> MSHHHHHHVSKIFFEQGTYQCLENCGTVALTIIRRGGDLTNTVFVDFRTEDGTANAGSDYEFTEGTVVFKPGETQKEIRVGIIDDDIFEEDKNFLVHLSNVKVSSEASEDGILEANHVSALACLGSPSTATVTIFDDDHAGIFTFEEPVTHVSESIGIMEVKVLRTSGARGNVIVPYKTIEGTARGGGEDFEDTCGELEFQNDEIVKTISVKVIDDEEYEKNKTFFLEIGEPRLVEMSEKKGGFTITEEYDDKQPLTSKEEEERRIAEMGRPILGEHTKLEVIIEESYEFKSTVD

In contrast, the eukaryotic NCX has evolved an allosteric Ca2+ regulatory element encoded by a large cytosolic domain (∼500 amino acids) between transmembrane helices 5 and 6 i.e. the repeated membrane motif, designated as f-loop. This large loop includes two Ca2+-binding regulatory domains (CBD1 and CBD2), connected by a short linker. High-resolution NMR and crystal structures of isolated CBD1 and CBD2 domains of eukaryotic NCX revealed four Ca2+ sites (Ca1-Ca4) on CBD1 and two Ca2+ sites (CaI-CaII) on CBD2. Different lines of evidence suggest that CBD2 interacts with CBD1 to modify the equilibrium and kinetic properties of the primary Ca2+ sensor (Ca3-Ca4 sites), either in isolated CBD12 or in intact NCX.

To test this working hypothesis, we crystallized and determined the crystal structure of a two-domain CBD12 tandem from the brain splice variant (NCX1.4). In order to crystallize the tandem, we employed a previously characterized mutant, E454K. (i) The E454K substitution replaces the Ca2+ ion at Ca1 site of CBD1, thus, stabilizing the protein’s structure through a charge compensation mechanism. The overall structure of CBD12-E454K shows two nearly identical CBD domains, each composed of an anti-parallel β-sandwich, with root mean square deviation (r.m.s.d for 109 Cα atoms) of 1.3 Å. In agreement with the previously published crystal structure of CBD1-E454K, our structure reveals three Ca2+ ions in CBD1 that correspond to Ca2, Ca3 and Ca4 in CBD1-WT. Notably, there is no indication for bound Ca2+ ions in CBD2 of our structure. We ascribe the lack of bound Ca2+ in CBD2 to crystal packing between symmetry mates. The interface involves mainly interactions of the CBD1 Ca2+ binding loops with the interdomain linker, the CBD2 flexible FG loop and the strictly conserved CBD2 BC loop. The first hydrophilic region includes a pivotal interdomain electrostatic network centered at R532 in CBD2. This arginine takes a conformation that forms bifurcated hydrogen-bonded and non-hydrogen-bonded salt-bridges with D499, D500 in CBD1 and D565 in CBD2.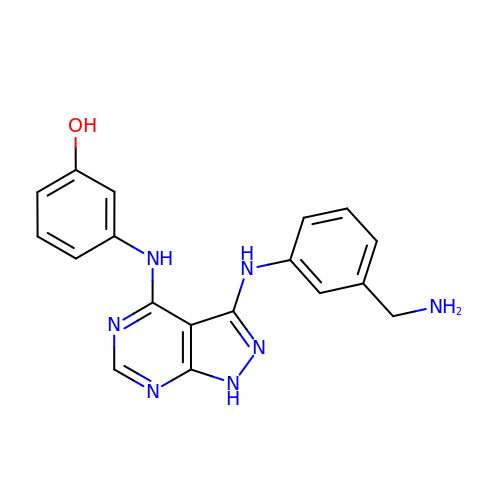3-[[3-[[3-(aminomethyl)phenyl]amino]-1~{H}-pyrazolo[3,4-d]pyrimidin-4-yl]amino]phenol | C18 H17 N7 O | OUMZUIUUJCKLOT-UHFFFAOYSA-N> MAHAGRTGYDNREIVMKYIHYKLSQRGYEWDAGDDVEENRTEAPEGTESEVVHLTLRQAADDFSRRYRRDFAEMSSQLHLTPFTARGRFATVVEELFRDGVNWGRIVAFFEFGGVMCVESVNREMSPLVDNIALWMTEYLNRHLHTWIQDNGGWDAFVELYGPSMR

BCL-2 is the founding member of the pro-survival class of proteins that includes BCL-XL, BCL-W, A1/BFL-1 and MCL-1. They exert their pro-survival function by binding and restraining related members of a family of pro-apoptotic proteins—the sensors of cellular stress (the BH3-only proteins) and the effectors of apoptosis (BAX and BAK). Four or more hydrophobic amino acids on successive helical turns within the BH3 motif engage complementary pockets (P1 through P4) in this surface groove of pro-survival proteins. Venetoclax competes with pro-apoptotic BH3 motifs for BCL-2 binding, releasing pro-apoptotic proteins and allowing apoptosis in cells primed for death.

Additionally, we obtained a structure of BCL-2 G101A bound to venetoclax, representing a milder introduction of bulk at the G101 position than the valine substitution. The BCL-2 G101A:venetoclax and BCL-2 WT:venetoclax crystals were isomorphous and there were no significant deviations in venetoclax positioning or E152. Furthermore, the E152 conformation in a BCL-2 G101A:venetoclax structure matched the WT conformation, not the G101V. The G101A mutant bound to venetoclax with a KI of 110 pM comparable to WT but distinct from G101V. Additionally, introduction of an alanine at the G101 position did not provide sufficient bulk to displace E152 in the crystal structure and affinity for venetoclax was maintained for the G101A mutant.>[2x]MNTTPVHALTDIDGGIAVDPAPRLAGPPVFGGPGNDAFDLAPVRSTGREMLRFDFPGVSIGAAHYEEGPTGATVIHIPAGARTAVDARGGAVGLSGGYDFNHAICLAGGAGYGLEAGAGVSGALLERLEYRTGFAELQLVSS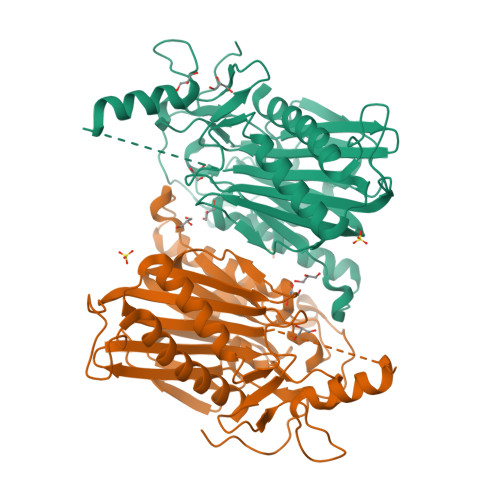AVIYDFSARSTAVYPDKALGRAALEFAVPGEFPQGRAGAGMSASAGKVDWDRTEITGQGAAFRRLGDVRILAVVVPNPVGVIVDRAGTVVRGNYDAQTGVRRHPVFDYQEAFAEQVPPVTEAGNCTISAIVTNVRMSPVELNQFAKQVHSSMHRGIQPFHTDMDGDTLFAVTTDEIDLPTTPGSSRGRLSVNATALGAIASEVMWDAVLEAGK> MHHHHHHSSGRENLYFQGHMYK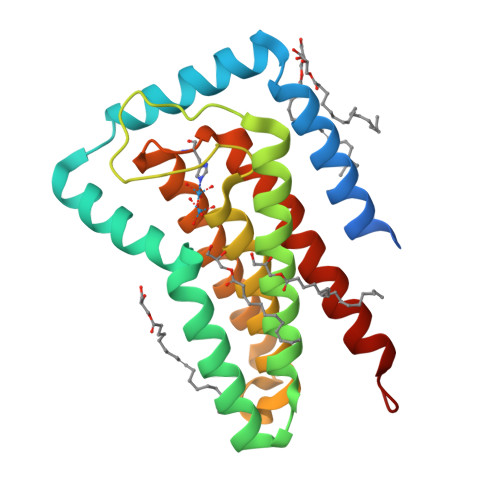PVSLFLFFLILAAAIHTNAVQSADEAISKAAVLIRQPWLNEVMTGITHLGASSFLLPLIVIIGAGMFFYRKTWDGLLMLLVFGTDRLLNKVLKEWIERVRPDFAPLVHESSFSFPSGHSMNAACVYPVIAYFLVKHLPFLSKHKKMVYIIAGVIAVLVGISRVYLGVHFVTDVLGGFSLGLLLFFLVKGFDEKIKRFRQK> SHMREESLQLMDLLGLERSAWGNIPLMRKAYLKKCKEFHPD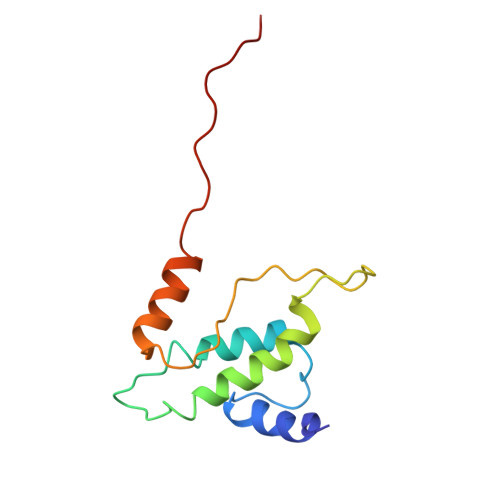KGGDEEKMKKMNTLYKKMEDGVKYAHQPDFGGFWDATEIPTYGTDEWEQWWNAFNEENLFCSEEMPSSDDEAT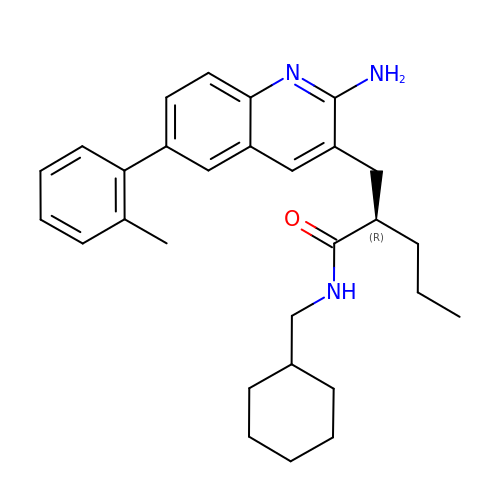(2R)-2-{[2-amino-6-(2-methylphenyl)quinolin-3-yl]methyl}-N-(cyclohexylmethyl)pentanamide | C29 H37 N3 O | KSRGIPYZQZCBMH-HSZRJFAPSA-N ethyl 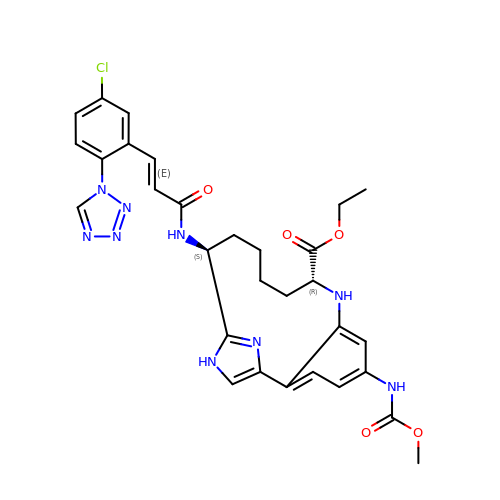(2R,7S)-7-({(2E)-3-[5-chloro-2-(1H-tetrazol-1-yl)phenyl]prop-2-enoyl}amino)-14-[(methoxycarbonyl)amino]-1,2,3,4,5,6,7,9-octahydro-11,8-(azeno)-1,9-benzodiazacyclotridecine-2-carboxylate | C30 H32 Cl N9 O5 | BNKJNEZXZHRTHJ-GGRGIUQZSA-N The RecBCD complex of Escherichia coli plays a dual role in bacterial cell biology, acting both as a phage immunity hub and as the primary mechanism to initiate the recombinational repair of double-stranded DNA breaks (DSBs). The switch from the destructive to the recombinogenic mode is triggered during RecBCD translocation along DNA by recognition of a specific octameric ssDNA sequence called Chi (crossover hotspot instigator; 5′-GCTGGTGG-3′). Here, we present biochemical and structural analysis of two phage proteins, gp5.9 and Abc2, which target the DNA break resection complex RecBCD. These exemplify two contrasting mechanisms for control of DNA break repair in which the RecBCD complex is either inhibited or co-opted for the benefit of the invading phage.

We next purified the RecBCD-gp5.9 complex (using the tag-free form of gp5.9) and analysed its structure using single-particle cryoEM. There was structural heterogeneity only within the RecD protein, suggesting that the RecD conformation becomes uncoupled to the rest of the complex when bound to gp5.9. A 3.2 Å resolution cryoEM map was obtained facilitating the building of a model for two chains of gp5.9, both containing residues 1–49. The structure reveals that gp5.9 adopts a parallel coiled-coil architecture in which the N-termini are slightly braced apart by a short anti-parallel beta-sheet. Many aspartate and glutamate residues are displayed on the outer surface of this exceptionally negatively charged protein (pI = 4.0). The phage protein engages RecBCD in a position which overlaps extensively with the DNA binding site and also with the binding site for the DNA mimic protein Gam. The C-terminal end of the coiled-coil binds to the extended RecB arm domain, while the N-terminus binds closer to the RecBCD core, making contacts with both the RecB and RecC subunits and helping to explain the reduced efficacy of inhibition by purified gp5.9 retaining an N-terminal tag. The overall structures of RecBCD when bound to either DNA or gp5.9 are almost identical, although small rigid body domain movements help accommodate differences in the dimensions of the two ligands. Many ion pair contacts are formed between D/E and K/R residues in gp5.9 and RecBCD, respectively. These imitate a subset of the contacts formed between the negatively charged DNA phosphates and K/R residues in the RecBCD-DNA complex and, on this basis, we can conclude that gp5.9 acts by DNA mimicry.

> MSDVAETLDPLRLPLQGERLIEASAGTGKTFTIAALYLRLLLGLGGSAAFPRPLTVEELLVVTFTEAATAELRGRIRSNIHELRIACLRETTDNPLYERLLEEIDDKAQAAQWLLLAERQMDEAAVFTIHGFCQRMLNLNAFESGMLFEQQLIEDESLLRYQACADFWRRHCYPLPREIAQVVFETWKGPQALLRDINRYLQGEAPVIKAPPPDDETLASRHAQIVARIDTVKQQWRDAVGELDALIESSGIDRRKFNRSNQAKWIDKISAWAEEETNSYQLPESLEKFSQRFLEDRTKAGGETPRHPLFEAIDQLLAEPLSIRDLVITRALAEIRETVAREKRRRGELGFDDMLSRLDSALRSESGEVLAAAIRTRFPVAMIDEFQDTDPQQYRIFRRIWHHQPETALLLIGDPKQAIYAFRGADIFTYMKARSEVHAHYTLDTNWRSAPGMVNSVNKLFSQTDDAFMFREIPFIPVKSAGKNQALRFVFKGETQPAMKMWLMEGESCGVGDYQSTMAQVCAAQIRDWLQAGQRGEALLMNGDDARPVRASDISVLVRSRQEAAQVRDALTLLEIPSVYLSNRDSVFETLEAQEMLWLLQAVMTPERENTLRSALATSMMGLNALDIETLNNDEHAWDVVVEEFDGYRQIWRKRGVMPMLRALMSARNIAENLLATAGGERRLTDILHISELLQEAGTQLESEHALVRWLSQHILEPDSNASSQQMRLESDKHLVQIVTIHKSKGLEYPLVWLPFITNFRVQEQAFYHDRHSFEAVLDLNAAPESVDLAEAERLAEDLRLLYVALTRSVWHCSLGVAPLVRRRGDKKGDTDVHQSALGRLLQKGEPQDAAGLRTCIEALCDDDIAWQTAQTGDNQPWQVNDVSTAELNAKTLQRLPGDNWRVTSYSGLQQRGHGIAQDLMPRLDVDAAGVASVVEEPTLTPHQFPRGASPGTFLHSLFEDLDFTQPVDPNWVREKLELGGFESQWEPVLTEWITAVLQAPLNETGVSLSQLSARNKQVEMEFYLPISEPLIASQLDTLIRQFDPLSAGCPPLEFMQVRGMLKGFIDLVFRHEGRYYLLDYKSNWLGEDSSAYTQQAMAAAMQAHRYDLQYQLYTLALHRYLRHRIADYDYEHHFGGVIYLFLRGVDKEHPQQGIYTTRPNAGLIALMDEMFAGMTLEEA;> MLRVYHSNRLDVLEALMEFIVERERLDDPFEPEMILVQSTGMAQWLQMTLSQKFGIAANIDFPLPASFIWDMFVRVLPEIPKESAFNKQSMSWKLMTLLPQLLEREDFTLLRHYLTDDSDKRKLFQLSSKAADLFDQYLVYRPDWLAQWETGHLVEGLGEAQAWQAPLWKALVEYTHQLGQPRWHRANLYQRFIETLESATTCPPGLPSRVFICGISALPPVYLQALQALGKHIEIHLLFTNPCRYYWGDIKDPAYLAKLLTRQRRHSFEDRELPLFRDSENAGQLFNSDGEQDVGNPLLASWGKLGRDYIYLLSDLESSQELDAFVDVTPDNLLHNIQSDILELENRAVAGVNIEEFSRSDNKRPLDPLDSSITFHVCHSPQREVEVLHDRLLAMLEEDPTLTPRDIIVMVADIDSYSPFIQAVFGSAPADRYLPYAISDRRARQSHPVLEAFISLLSLPDSRFVSEDVLALLDVPVLAARFDITEEGLRYLRQWVNESGIRWGIDDDNVRELELPATGQHTWRFGLTRMLLGYAMESAQGEWQSVLPYDESSGLIAELVGHLASLLMQLNIWRRGLAQERPLEEWLPVCRDMLNAFFLPDAETEAAMTLIEQQWQAIIAEGLGAQYGDAVPLSLLRDELAQRLDQERISQRFLAGPVNICTLMPMRSIPFKVVCLLGMNDGVYPRQLAPLGFDLMSQKPKRGDRSRRDDDRYLFLEALISAQQKLYISYIGRSIQDNSERFPSVLVQELIDYIGQSHYLPGDEALNCDESEARVKAHLTCLHTRMPFDPQNYQPGERQSYAREWLPAASQAGKAHSEFVQPLPFTLPETVPLETLQRFWAHPVRAFFQMRLQVNFRTEDSEIPDTEPFILEGLSRYQINQQLLNALVEQDDAERLFRRFRAAGDLPYGAFGEIFWETQCQEMQQLADRVIACRQPGQSMEIDLACNGVQITGWLPQVQPDGLLRWRPSLLSVAQGMQLWLEHLVYCASGGNGESRLFLRKDGEWRFPPLAAEQALHYLSQLIEGYREGMSAPLLVLPESGGAWLKTCYDAQNDAMLDDDSTLQKARTKFLQAYEGNMMVRGEGDDIWYQRLWRQLTPETMEAIVEQSQRFLLPLFRFNQS;> MKLQKQLLEAVEHKQLRPLDVQFALTVAGDEHPAVTLAAALLSHDAGEGHVCLPLSRLENNEASHPLLATCVSEIGELQNWEECLLASQAVSRGDEPTPMILCGDRLYLNRMWCNERTVARFFNEVNHAIEVDEALLAQTLDKLFPVSDEINWQKVAAAVALTRRISVISGGPGTGKTTTVAKLLAALIQMADGERCRIRLAAPTGKAAARLTESLGKALRQLPLTDEQKKRIPEDASTLHRLLGAQPGSQRLRHHAGNPLHLDVLVVDEASMIDLPMMSRLIDALPDHARVIFLGDRDQLASVEAGAVLGDICAYANAGFTAERARQLSRLTGTHVPAGTGTEAASLRDSLCLLQKSYRFGSDSGIGQLAAAINRGDKTAVKTVFQQDFTDIEKRLLQSGEDYIAMLEEALAGYGRYLDLLQARAEPDLIIQAFNEYQLLCALREGPFGVAGLNERIEQFMQQKRKIHRHPHSRWYEGRPVMIARNDSALGLFNGDIGIALDRGQGTRVWFAMPDGNIKSVQPSRLPEHETTWAMTVHKSQGSEFDHAALILPSQRTPVVTRELVYTAVTRARRRLSLYADERILSAAIATRTERRSGLAALFSSRE;>[2x]MSRDLVTIPRDVWNDIQGYIDSLERENDSLKNQLMEADEYVAELEEKLNGTS>MNTTPVHALTDIDGGIAVDPAPRLAGPPVFGGPGNDAFDLAPVRSTGREMLRFDFPGVSIGAAHYEEGPTGATVIHIPAGARTAVDARGGAVGLSGGYDFNHAICLAGGAGYGLE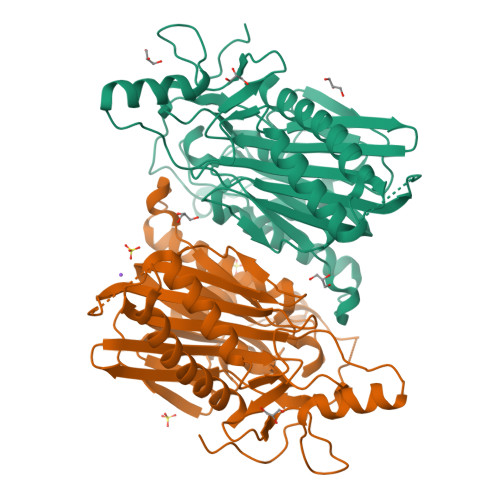AGAGVSGALLERLEYRTGFAELQLVSSAVIYDFSARSTAVYPDKALGRAALEFAVPGEFPQGRAGAGMSASAGKVDWDRTEITGQGAAFRRLGDVRILAVVVPNPVGVIVDRAGTVVRGNYDAQTGVRRHPVFDYQEAFAEQVPPVTEAGNCTISAIVTNVRMSPVELNQFAKQVHSSMHRGIQPFHTDMDGDTLFAVTTDEIDLPTTPGSSRGRLSVNATALGAIASEVMWDAVLEAGK[2x]>MTVQAQNIDAITAGAMPHEEPELTDGFHLVIDALKLNGIETIYNVPGIPITDLGRLAQAEGLRVISFRHEQNAGNAAAIAGFLTKKPGICLTVSAPGFLNGLTALANATTNCFPMILISGSSEREIVDLQQGDYGEMDQLAIAKPLCKAAFRVLHAADIGIGVARAIRAAVSGRPGGVYLDLPAKLFSQVIDADLGARSLVKVIDAAPAQLPAPAAIARALDVLKSAERPLIILGKGAAYAQADEAVRALVEESGIPYVPMSMAKGLLPDTHPLSAGAARSTALKDSDVVLLVGARLNWLLSHGKGKTWGEPGSKRFIQIDIEPREMDSNVEIVAPVVGDIGSCVEALLDGIRKDWKGAPSNWLETLRGKREANIAKMAPKLMKNSSPMCFHSALGALRTVIKERPDAILVNEGCNTLDLARGIIDMYQPRKRLDVGTWGVMGIGMGFAVAAAVETGKPVLAVEGDSAFGFSGMEVETICRYELPVCIVIFNNNGIFRGTDTDPTGRDPGTTVFVKNSRYDKMMEAFGGVGVNVTTPDELKRAVDEAMNSGKPTLINAEIDPAAGSEGGNIGSLNPQSTLKKK[8x]

Here, we employed structure-guided iterative saturation mutagenesis to convert oxalyl-CoA decarboxylase (OXC) from Methylobacterium extorquens into a glycolyl-CoA synthase (GCS) that allows for the direct condensation of the two C1 units formyl-CoA and formaldehyde. Previously, we showed that besides the decarboxylation of oxalyl-CoA into formyl-CoA, OXC from Methylorubrum extorquens (MeOXC) is also capable of catalyzing the acyloin condensation of formyl-CoA with various aldehydes, including formaldehyde. During catalysis, OXC and HACL both form the same α-carbanion/enamine intermediate. In HACL, this intermediate is generated through proton abstraction from formyl-CoA or by cleaving off the aldehyde moiety from a 2-hydroxyacyl-CoA thioester, whereas in OXC, this intermediate is formed by decarboxylation of oxalyl-CoA.

Thus, after screening ∼3600 clones in six rounds, we obtained the final variant MeOXC4 carrying four substitutions E135G, A415C, Y497F, and S568G. To rationalize the effect of the different substitutions on catalysis, we solved the crystal structure of MeOXC4 to a resolution of 2.4 Å, modeled its flexible C-terminus beyond E567 and compared it to MeOXC WT and OfOXC. Structural analysis showed that C415 is in close proximity to S568 of the flexible C-terminal loop reaching the active site, suggesting that this substitution is important to (re-)organize the active site for the new substrate. Substitution S568G lies within the flexible C-terminal loop, adjacent to A415C, and likely provides space to accommodate the bulkier side chain of C415. The third substitution E135G caused the greatest structural change by creating an extra cavity at the active site. Thus, the E135G substitution does not serve in substrate accommodation but likely allows optimal positioning of Y134 during catalysis, which is supported by the fact that kcat increased approximately fourfold by the E135G substitution, while the apparent KM value for formyl-CoA slightly increased. Three-ordered water molecules (W1–3) are observed in a structure with a trapped α-carbanion/enamine intermediate, with W2 (in close contact to W1 and W3) proposed to protonate the Cα of the intermediate.28 W1 is hydrogen-bonded to residues corresponding to Y134 and E135, while Y497 and S568 form hydrogen bonds to W3.28 In MeOXC4, this hydrogen bonding network to W1 and W3 is lost due to the E135G, Y497F, and S568G substitutions. This change in the water network likely helps to promote GCS activity at the expense of the OXC reaction. In summary, our structural analysis showed that the active site of MeOXC4 is reorganized for improved substrate accommodation and increased catalytic activity.>DYKDDDDKSHSPHLPRPHSRVPPHPSSERRAVYIGALFPMSGGWPGGQACQPAVEMALEDVNSRRDILPDYELKLIHHDSKCDPGQATKYLYELLYNDPIKIILMPGCSSVSTLVAEAARMWNLIVLSYGSSSPALSNRQRFPTFFRTHPSATLHNPTRVKLFEKWGWKKIATIQQTTEVFTSTLDDLEERVKEAGIEITFRQSFFSDPAVPVKNLKRQDARIIVGLFYETEARKVFCEVYKERLFGKKYVWFLIGWYADNWFKIYDPSINCTVDEMTEAVEGHITTEIVMLNPANTR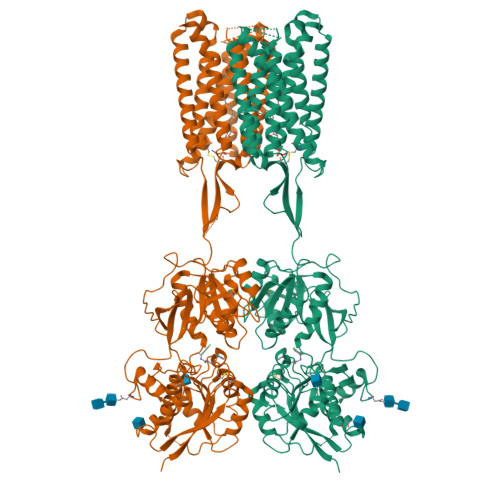SISNMTSQEFVEKLTKRLKRHPEETGGFQEAPLAYDAIWALALALNKTSGGGGRSGVRLEDFNYNNQTITDQIYRAMNSSSFEGVSGHVVFDASGSRMAWTLIEQLQGGSYKKIGYYDSTKDDLSWSKTDKWIGGSPPADQTLVIKTFRFLSQKLFISVSVLSSLGIVLAVVCLSFNIYNSHVRYIQNSQPNLNNLTAVGCSLALAAVFPLGLDGYHIGRNQFPFVCQARLWLLGLGFSLGYGSMFTKIWWVHTVFTKKEEKKEWRKTLEPWKLYATVGLLVGMDVLTLAIWQIVDPLHRTIETFAKEEPKEDIDVSILPQLEHCSSRKMNTWLGIFYGYKGLLLLLGIFLAYETKSVSTEKINDHRAVGMAIYNVAVLCLITAPVTMILSSQQDAAFAFASLAIVFSSYITLVVLFVPKMRRLITRGEWQSEAQDTMKTGSSTNNNEEEKSRLLEKENRELEKIIAEKEERVSELRHQLQSRQQLRSRRHPPTPPEPSGGLPRGPPEPPDRLSCDGSRVHLLYKHHHHHH[2x]>GQFKRIALLGMPNTGKSTLFNRMTGGAARVGNWPGITVELLSGKILLGADMVEIIDLPGIYDLHGFSDDEQVVRHFLHDNVPDLALVILNATQIERQMSLLLQLKQLNMNIVVLLNMSDEAKQYGITIDSRKMSELLQIPVFQLSGKYGTGYQ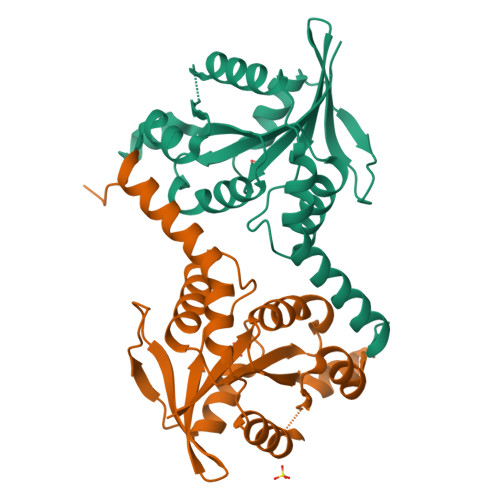EALQAVTRALRYPTPGMAENVRTQLEQDEHIEAEMVRILKSAVQIPARLPE[2x]> MDYKDDDDKRSPVRDLARNDGEESTDRTPLLPGAPRAEAAPVCCSARYNLAILAFFGFFIVYALRVNLSVALVDMVDSNTTLEDNRTSKACPEHSAPIKVHHNQTGKKYQWDAETQGWILGSFFYGYIITQIPGGYVASKIGGKMLLGFGILGTAVLTLFTPIAADLGVGPLIVLRALEGLGEGVTFPAMHAMWSSWAPPLERSKLLSISYAGAQLGTVISLPLSGIICYYMNWTYVFYFFGTIGIFWFLLWIWLVSDTPQKHKRISHYEKEYILSSLRNQLSSQKSVPWVPILKSLPLWAIVVAHFSYNWTFYTLLTLLPTYMKEILRFNVQENGFLSSLPYLGSWLCMILSGQAADNLRAKWNFSTLCVRRIFSLIGMIGPAVFLVAAGFIGCDYSLAVAFLTISTTLGGFCSSGFSINHLDIAPSYAGILLGITNTFATIPGMVGPVIAKSLTPDNTVGEWQTVFYIAAAINVFGAIFFTLFAKGEVQNWALNDHHGHRH

Sialin, a member of the solute carrier 17 (SLC17) transporter family, is unique in its ability to transport not only sialic acid using a pH-driven mechanism, but also transport mono and diacidic neurotransmitters, such as glutamate and N-acetylaspartylglutamate (NAAG), into synaptic vesicles via a membrane potential-driven mechanism. Sialin (SLC17A5) belongs to the solute carrier 17 (SLC17) transporter subfamily that includes nine related transmembrane major facility superfamily (MFS) transporters, all of which are dedicated to anion transport, including the vesicular glutamate transporters 1-3 (VGLUT1–3) and a vesicular nucleotide transporter (VNUT). Sialin adopts a classical MFS fold consisting of 12 transmembrane helices (TMs) with two pseudo-symmetric domains: N-domain (TMs 1-6) and C-domain (TMs 7-12). The Sialin structures in both the lumen-open and cytosol-open conformations reveal a solvent-accessible cavity, which forms the substrate translocation pathway, at the center of the interface between the N-domain and C-domain.

The cryo-EM structures of SialinWT in the apo state were determined at 3.2-Å (pH 5.0) and 2.8-Å (pH 7.5) resolution respectively. The overall structure of SialinWT has the same fold with the recently determined cytosol-open structure of human Sialin19, with a root mean square deviation (R.M.S.D.) value of 0.5 Å. In the cytosol-open state, Phe116 on TM2 forms π-π interaction with Tyr306 on TM7 and Gln123 on TM2 interacts with Thr434 on TM11, leading to a collapse of the translocation pathway in the luminal leaflet. The interaction between Tyr335 on TM8 and Leu309 on TM7 ensures that Leu309 is in a certain conformation to interact with Val58 and Ser61 on TM1 to further lock Sialin in the cytosol-open state. Since Arg39 forms a salt bridge with Glu262 and Lys136 binds to the carbonyl of Val248, two Salla disease-causing mutations (Arg39Cys and Lys136Glu) destabilize the cytosolic opening of Sialin.>GQDMVSPPPPIADEPLTVN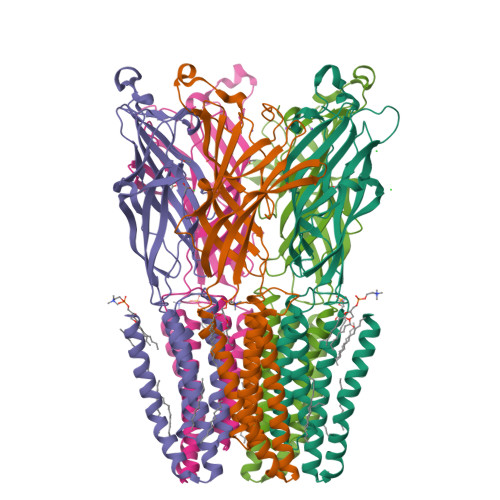TGIYLIECYSLDDKAETFKVNAFLSLSWKDRRLAFDPVRSGVRVKTYEPEAIWIPEIRFVNVENARDADVVDISVSPDGTVQYLERFSARVLSPLDFRRYPFDSQTLHIYLIVRSVDTRNIVLAVDLEKVGKNDDVFLTGWDIESFTAVVKPANFALEDRLESKLDYQLRISRQYFSYIPNIILPMLFILFISWTAFWSTSYEANVTLVVSTLIAHIAFNILVETNLPCTPYMTYTGAIIFMIYLFYFVAVIEVTVQHYLKVESQPARAASITRASRIAFPVVFLLANIILAFLFFGF[5x]> MILTITYTQPPATDLGYLLHKNPSRPQTFELNHGKAHIFYPEATSERCTVALLLDIDPIDLARGKKGSSGEGGLFDYVNDRPYVSSSFMSVAISRVFGTAMSGKCKEKPE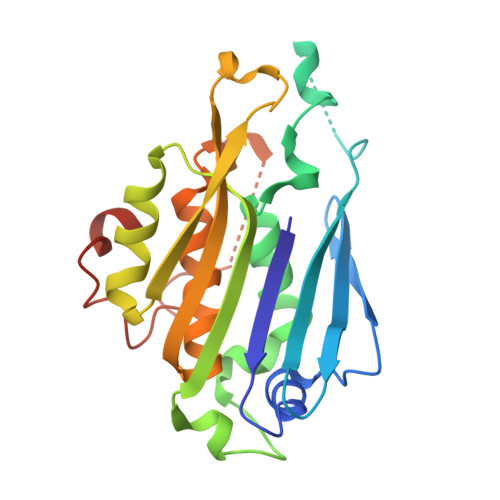LAAIKLPLKAKIMMLPCKGGEEIIYRLFEPLGYKVDVEGYMLDEKFPEWGKSRYYTVSLEGEVRVRDLLNHIYVLIPVLDSEKHYWVGEDEIDKLFQHGEGWLVDHPEKELITGRYLIRK> MPRPSLYEILYGNFTGGLELNQVGEEEQVILSVLDNMQRILNTRAGSLKHLPDYGLPDITTILQGMPGTAHQLMRVLSDVLL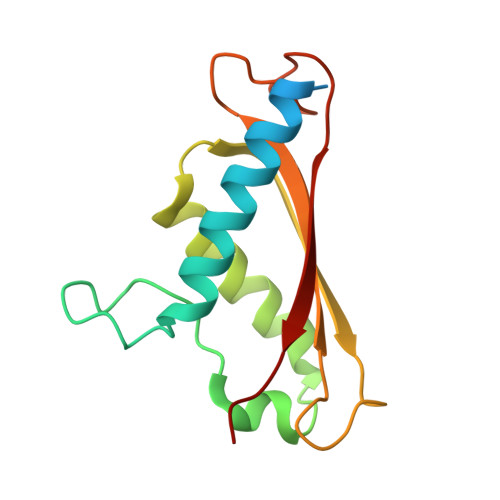KYEPRIKRVDVTMQEQTQPGELHYVIDAELKDAGLVRYGTTFIPEGRVLLRHLKQQRYVQT> GPHMAESHLQSSLITASQFFEIWLHFDADGSGYLEGKELQNLIQELQQARKKAGLELSPEMKTFVDQYGQRDDGKIGIVELAHVLPTEENFLLLFRCQQLKSCEEFMKTWRKYDTDHSGFIETEELKNFLKDLLEKANKTVDDTKLAEYTDLMLKLFDSNNDGKLELTEMARLL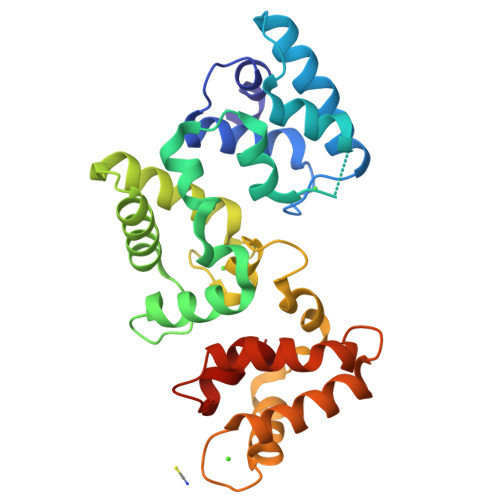PVQENFLLKFQGIKMCGKEFNKAFELYDQDGNGYIDENELDALLKDLCEKNKQDLDINNITTYKKNIMALSDGGKLYRTDLALILCAGDN>[2x]GASGDLYEVERIVDKRKNKKGKWEYLIRWKGYGSTE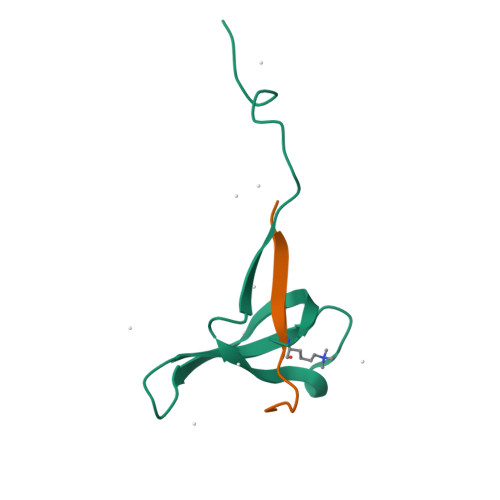DTWEPEHHLLHCEEFIDEFNGLHMSKDK;>XQLATKAARKSAPATYX[2x]>MDIKINDITLGNNSPFVLFGGI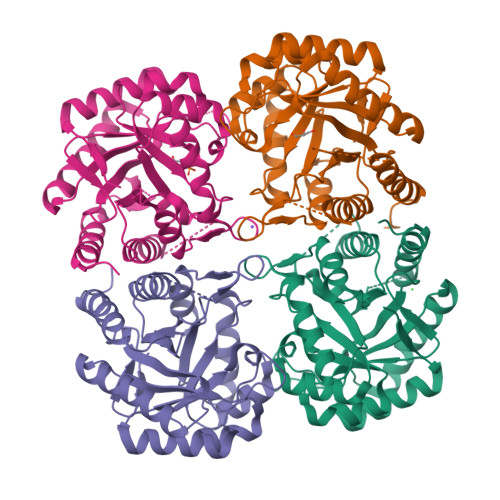CVLESLDSTLQTCAHYVEVTRKLGIPYIFKASFDKANRSSIHSYRGVGLEEGLKIFEKVKAEFGIPVITDVHEPHQCQPVAEVCDVIQLPAFLARQTDLVVAMAKTGNVVNIKKPQFLSPSQMKNIVEKFHEAGNGKLILCERGSSFGYDNLVVDMLGFGVMKQTCGNLPVIFDVTHSLQTRDAGSAASGGRRAQALDLALAGMATRLAGLFLESHPDPKLAKSEGASALPLHLLEDFLIRIKALDDLIKSQPILTIE[4x]>SLLNVPAGKDLPEDIYVVIEIPANADPIKYEIDKESGALFVDRFMSTAMFYPCNYGYINHTLSLDGDPVDVLVPTPYPLQPGSVTRCRPVGVLKMTDEAG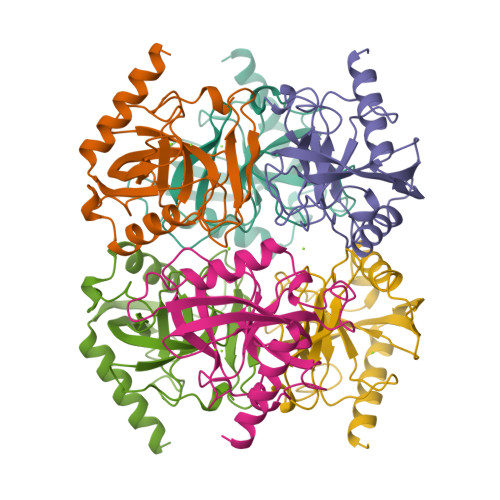EDAKLVAVPHSKLSKEYDHIKDVNDLPELLKAQIAHFFEHYKDLEKGKWVKVEGWENAEAAKAEIVASFERAKNK[3x]>[2x]RSPGTLPRKAGVFSDLSNQELKAVHSFLWSKKELRLQPSSTTTMAKNTVFLIEMLLP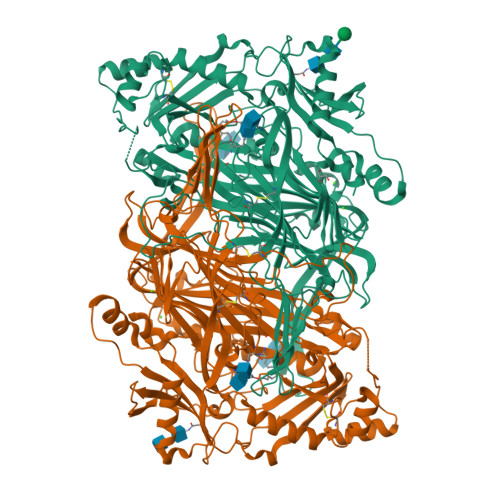KKYHVLRFLDKGERHPVREARAVIFFGDQEHPNVTEFAVGPLPGPCYMRALSPRPGYQSSWASRPISTAEYALLYHTLQEATKPLHQFFLNTTGFSFQDCHDRCLAFTDVAPRGVASGQRRSWLIIQRYVEGYFLHPTGLELLVDHGSTDAGHWAVEQVWYNGKFYGSPEELARKYADGEVDVVVLEDPLPGGKGHDSTEEPPLFSSHKPRGDFPSPIHVSGPRLVQPHGPRFRLEGNAVLYGGWSFAFRLRSSSGLQVLNVHFGGERIAYEVSVQEAVALYGGHTPAGMQTKYLDVGWGLGSVTHELAPGIDCPETATFLDTFHYYDADDPVHYPRALCLFEMPTGVPLRRHFNSNFKGGFNFYAGLKGQVLVLRTTSTVYNYDYIWDFIFYPNGVMEAKMHATGYVHATFYTPEGLRHGTRLHTHLIGNIHTHLVHYRVDLDVAGTKNSFQTLQMKLENITNPWSPRHRVVQPTLEQTQYSWERQAAFRFKRKLPKYLLFTSPQENPWGHKRSYRLQIHSMADQVLPPGWQEEQAITWARYPLAVTKYRESELCSSSIYHQNDPWDPPVVFEQFLHNNENIENEDLVAWVTVGFLHIPHSEDIPNTATPGNSVGFLLRPFNFFPEDPSLASRDTVIVWPRDNGPNYVQRWIPEDRDCSMPPPFSYNGTYRPV> VHQVLYRALVSTKWLAESVRAGKVGPGLRVLDASW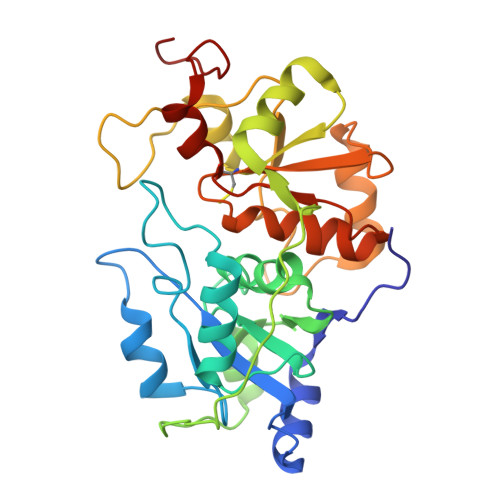YSPGTREARKEYLERHVPGASFFDIEECRDKASPYEVMLPSEAGFADYVGSLGISNDTHVVVYNGDDLGSFYAPRVWWMFRVFGHRTVSVLNGGFRNWLKEGHPVTSEPSRPEPAIFKATLNRSLLKTYEQVLENLESKRFQLVDSRAQGRYLGTQPEPDAVGLDSGHIRGSVNMPFMDFLTENGFEKSPEELRAMFEAKKVDLTKPLIATCRKGVTACHIALAAYLCGKPDVAIYDGSWFEWFHRAPPETWVSQGKG> MEGSIKEIAITHHVKEGHEKADPSQFELLKVLGQGSFGKVFLVKKISGSDARQLYAMKVLKKATLKVRDRVRTKMERDILVEVNHPFIVKLHYAFQTEGKLYLILDFLRGGDLFTRLSKEVMFTEEDVKFYLAELALALDHLHSLGIIYRDLKPENILLDEEGHIKLTDFGLSKESIDHEKKAYSFCGTVEYMAPEVVN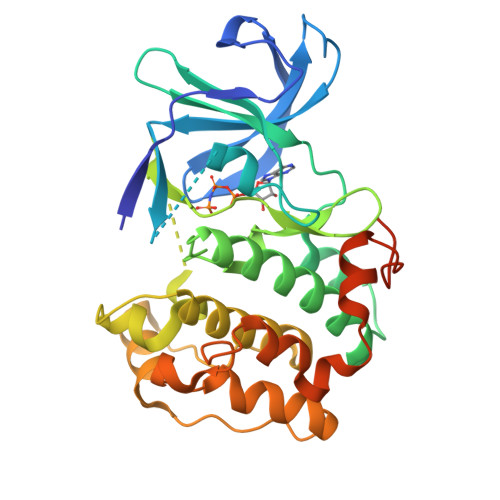RRGHTQSADWWSFGVLMFEMLTGTLPFQGKDRKETMTMILKAKLGMPQFLSPEAQSLLRMLFKRNPANRLGAGPDGVEEIKRHSFFSTIDWNKLYRREIHPPFKPATGRPEDTFYFDPEFTAKTPK N-[(1S,2R)-1-(3,5-difluorobenzyl)-2-hydroxy-3-({1-[3-(1H-pyrazol-1-yl)phenyl]cyclohexyl}amino)propyl]acetamide 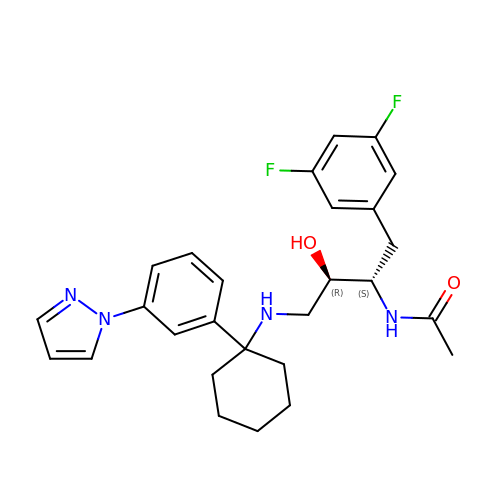| C27 H32 F2 N4 O2 | QXNFPOMRKODYSK-IZZNHLLZSA-N Here, we demonstrate that Rv3722c is the primary aspartate aminotransferase (AspAT) in Mtb, non-redundantly catalyzes the specific biosynthesis of Asp in vitro, and is essential for axenic growth and survival of Mtb in macrophages and in mice. The overall fold of Rv3722c is similar to that of other members of the recently described type Ic subgroup of PLP-binding proteins. Each monomer consists of a core domain (Pro52-Gly302) that folds into a nearly perfect α/β motif comprised a central eight-stranded (predominantly antiparallel) β-sheet surrounded by eight α-helices. Rv3722c also contains an N-terminal auxiliary domain (Ser2-Leu53 and Asp303-Ser430) that stacks and forms an elongated segment on top of the core domain, and consists of five α-helices and an antiparallel β-sheet.

To elucidate the structural basis of substrate recognition by Rv3722c, we have solved structures of the enzyme co-crystalized with Glu or Kyn at a resolution of 2.6 Å and 2.23 Å, respectively. The structure of Rv3722c pre-incubated with Glu demonstrated clear electron density of the amino acid in the active site located at the convergence of the auxiliary and core domain. Glu is engaged by both polar and nonpolar interactions. Canonical AspATs coordinate the side-chain carboxylate group of dicarboxylic substrates through a conserved active site Arg (or Lys). Our structure shows that Rv3722c also forms a salt bridge with side chain carboxylate group of Glu, but using a structurally non-homologous Arg residue at position 141.

>[4x]VSFDSLSPQELAALHARHQQDYAALQGMKLALDLTRGKPSAEQLDLSNQLLSLPGDDYRDPEGTDTRNYGGQHGLPGLRAIFAELLGIAVPNLIAGNNSSLELMHDIVAFSMLYGGVDSPRPWIQEQDGIKFLCPVPGYDRHFAITETMGIEMIPIPMLQDGPDVDLIEELVAVDPAIKGMWTVPVFGNPSGVTYSWETVRRLVQMRTAAPDFRLFWDNAYAVHTLTLDFPRQVDVLGLAAKAGNPNRPYVFASTSKITFAGGGVSFFGGSLGNIAWYLQYAGKKSIGPDKVNQLRHLRFFGDADGVRLHMLRHQQILAPKFALVAEVLDQRLSESKIASWTEPKGGYFISLDVLPGTARRTVALAKDVGIAVTEAGASFPYRKDPDDKNIRIAPSFPSVPDLRNAVDGLATCALLAATETLLNQGLASSAPNVR>AGQKVMITKMITDSVANPQMKQAFEQRLAKASTEDALNDIKRDIIRSAI[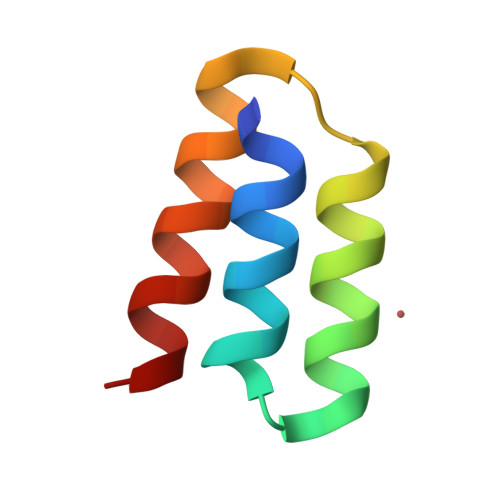2x]> MDPYCPFDALDVWEHRRFIVADSRNFITPEFPRDFWMSPVFNLPRETAAEQVVVLQAQRTAAAAALENAAMQAAELPVDIERRLRPIERNVHEIAGALEALETAAAAAEEADAARGDEPAGGGDGGAPPGLAVAEMEVQIVRNDPPLRYDTNLPVDLLHMVYAGRGATGSSGVVFGTWYRTIQDRTITDFPLTTRSADFRDGRMSKTFMTALVLSLQACGRLYVGQRHYSAFECAVLCLYLLYRNTHGAADDSDRAPVTFGDLLGRLPRYLACLAAVIGTEGGRPQYRYRDDKLPKTQFAAGGGRYEHGALASHIVIATLMHHGVLPAAPGDVPRDASTHVNPDGVAHHDDINRAAAAFLSRGHNLFLWEDQTLLRATANTITALGVIQRLLANGNVYADRLNNRLQLGMLIP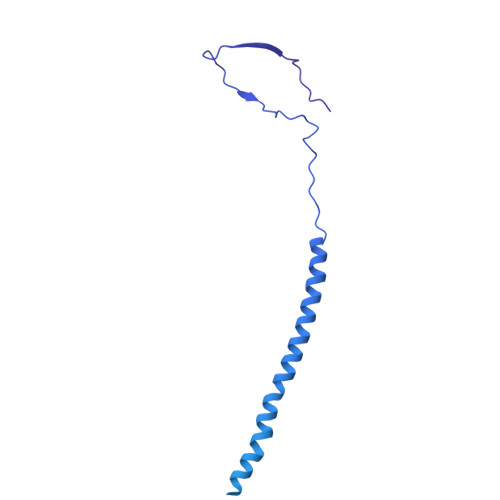GAVPSEAIARGASGSDSGAIKSGDNNLEALCANYVLPLYRADPAVELTQLFPGLAALCLDAQAGRPVGSTRRVVDMSSGARQAALVRLTALELINRTRTNPTPVGEVIHAHDALAIQYEQGLGLLAQQARIGLGSNTKRFSAFNVSSDYDMLYFLCLGFIPQYLSAV> MMSENKLHVIDLHKRYGGHEVLKGVSLQARAGDVISIIGSSGSGKSTFLRCINFLEKPSEGAIIVNGQNINLVRDKDGQLKVADKNQLRLLRTRLTMVFQHFNLWSHMTVLENVMEAPIQVLGLSKHDARERALKYLAKVGIDERAQGKYPVHLSGGQQQRVSIARALAMEPDVLLFDEPTSALDPELVGEVLRI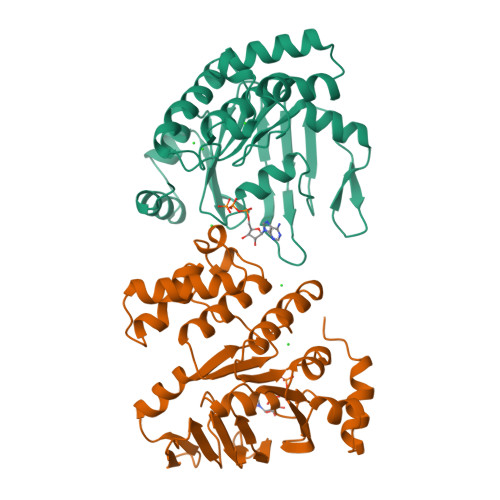MQQLAEEGKTMVVVTHEMGFARHVSSHVIFLHQGKIEEEGDPEQVFGNPQSPRLQQFLKGSLKKLEH> GPLGSMDINELIIGAQSADKHTREVAETQLLQWCDSDASQVFKALANVALQHEASLESRQFALLSLRKLITMYWSPGFESYRSTSNVEIDVKDFIREVLLKLCLNDNENTKIKNGASYCIVQISAVDFPDQWPQLLTVIYDAISHQHSLNAMSLLNEIYDDVVSEEMFFEGGIGLATMEIVFKVLNTETSTLIAKIAALKLLKACLLQMSSHNEYDEASRKSFVSQCLATSLQILGQLLTLNFGNVDVISQLKFKSIIYENLVFIKNDFSRKHFSSELQKQFKIMAIQDLENVTHINANVETTESEPLLETVHDCSIYIVEFLTSVCTLQFSVEEMNKIITSLTILCQLSSETREIWTSDFNTFVSKETGLAASYNVRDQANEFFTSLPNPQLSLIFKVVSNDIEHSTCNYSTLESLLYLLQCILLNDDEITGENIDQSLQILIKTLENILVSQEIPELILARAILTIPRVLDKFIDALPDIKPLTSAFLAKSLNLALKSDKELIKSATLIAFTYYCYFAELDSVLGPEVCSETQEKVIRIINQVSSDAEEDTNGALMEVLSQVISYNPKEPHSRKEILQAEFHLVFTISSEDPANVQVVVQSQECLEKLLDNINMDNYKNYIELCLPSFINVLDSNNANNYRYSPLLSLVLEFITVFLKKKPNDGFLPDEINQYLFEPLAKVLAFSTEDETLQLATEAFSYLIFNTDTRAMEPRLMDIMKVLERLLSLEVSDSAAMNVGPLVVAIFTRFSKEIQPLIGRILEAVVVRLIKTQNISTEQNLLSVLCFLTCNDPKQTVDFLSSFQIDNTDALTLVMRKWIEAFEVIRGEKRIKENIVALSNLFFLNDKRLQKVVVNGNLIPYEGDLIITRSMAKKMPDRYVQVPLYTKIIKLFVSELSFQSKQPNPEQLITSDIKQEVVNANKDDDNDDWED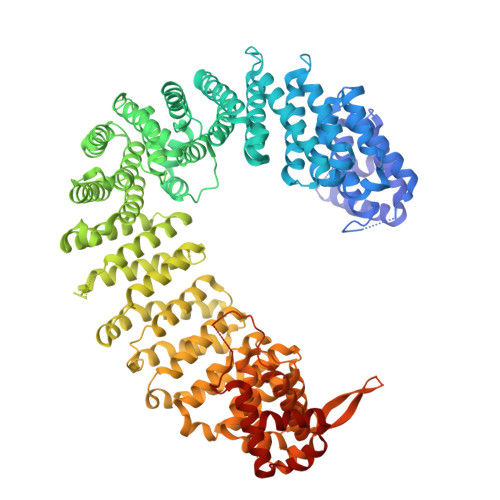VDDVLDYDKLKEYIDDDVDEEADDDSDDITGLMDVKESVVQLLVRFFKEVASKDVSGFHCIYETLSDSERKVLSEALL> GAAQPAMAQGALLQAQALYPWRAKKDNHLNFNKNDVITVLEQQ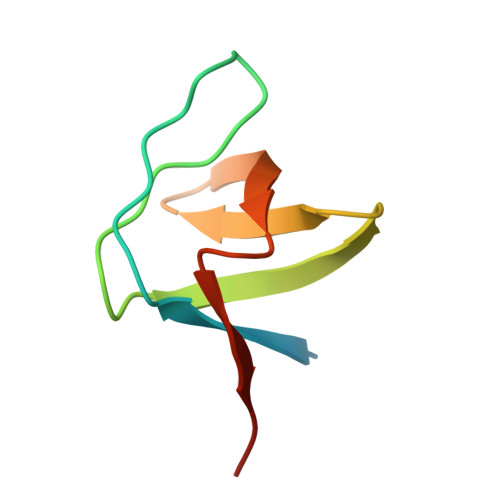DMWWFGEVQGQKGWFPKSYVKLISAAA4-(3-chloranyl-2-fluoranyl-phenoxy)-1-[[6-(1,3-thiazol-2-ylamino)pyridin-2-yl]methyl]cyclohexane-1-carboxylic acid | C22 H21 Cl F N3 O3 S | 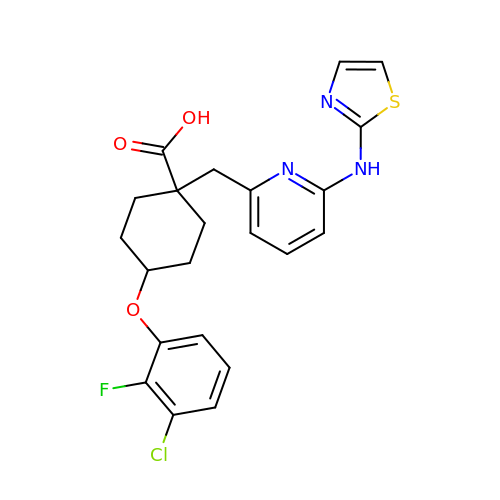LCVIRAZGMYMNNT-VVONHTQRSA-N>[2x]EAEAEFS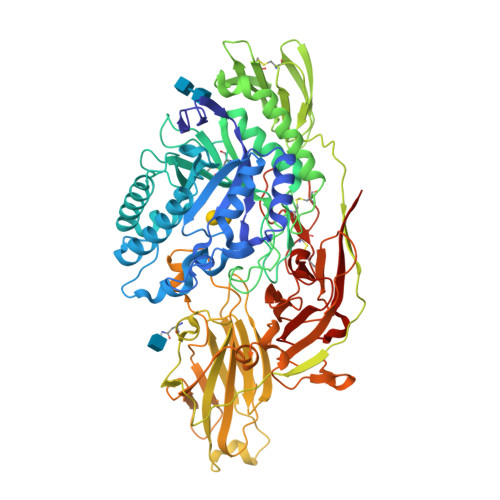VSYDDRAIIINGKRKILISGSIHYPRSTPQMWPDLIQKAKDGGLDVIETYVFWNGHEPSPGKYNFEGRYDLVRFIKMVQRAGLYVNLRIGPYVCAEWNFGGFPVWLKYVPGMEFRTNNQPFKVAMQGFVQKIVNMMKSENLFESQGGPIIMAQIENAYGPVEWEIGAPGKAYTKWAAQMAVGLKTGVPWIMCKQEDAPDPVIDTCNGFYCEGFRPNKPYKPKMWTEVWTGWYTKFGGPIPQRPAEDIAFSVARFVQNNGSFFNYYMYHGGTNFGRTSSGLFIATSYDYDAPLDEYGLLNEPKYGHLRDLHKAIKLSEPALVSSYAAVTSLGSNQEAHVYRSKSGACAAFLSNYDSRYSVKVTFQNRPYNLPPWSISILPDCKTAVYNTAQVNSQSSSIKMTPAGGGLSWQSYNEETPTADDSDTLTANGLWEQKNVTRDSSDYLWYMTNVNIASNEGFLKNGKDPYLTVMSAGHVLHVFVNGKLSGTVYGTLDNPKLTYSGNVKLRAGINKISLLSVSVGLPNVGVHYDTWNAGVLGPVTLSGLNEGSRNLAKQKWSYKVGLKGESLSLHSLSGSSSVEWVRGSLMAQKQPLTWYKATFNAPGGNDPLALDMASMGKGQIWINGEGVGRHWPGYIAQGDCSKCSYAGTFNEKKCQTNCGQPSQRWYHVPRSWLKPSGNLLVVFEEWGGNPTGISLVRRSRSAAAASFLEQK methyl [(2S)-1-{[(2R,6S,12Z,13aS,14aR,16aS)-2-[(7-methoxy-3-methylquinoxalin-2-yl)oxy]-14a-{[(1-methylcyclopropyl)sulfonyl]carbamoyl}-5,16-dioxo-1,2,3,5,6,7,8,9,10,11,13a,14,14a,15,16,16a-hexadecahydrocyclopropa[e]pyrrolo[1,2-a][1,4]diazacyclopentadecin-6-yl]amino}-3,3-dimethyl-1-oxobutan-2-yl]carbamate 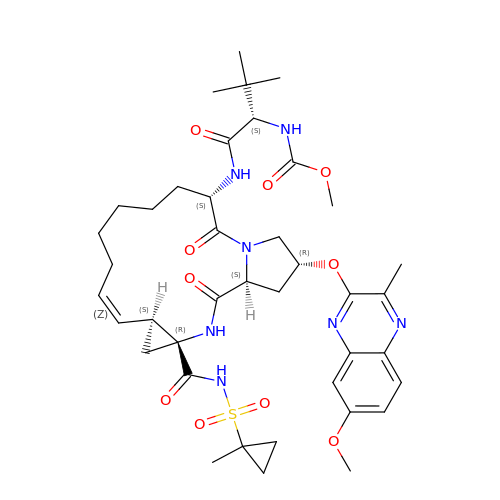| C40 H55 N7 O10 S | KNHVGXZTFPBTRE-VQPXEURISA-N> MRGSHHHHHHGMASEDRPIKFSTEGATSQSYKQFIEALRERLRGGLIHDIPVLPDPTTLQERNRYITVELSNSDTESIEVGIDVTNAYVVAYRAGTQSHFLRDAPSSASDYLFTGTDQHSLPFYGTYGDLERWAHQSRQQIPLGLQALTHGISFFRSGGNDNEEKARTLIVIIQMVAEAARFRYISNRVRVSIQT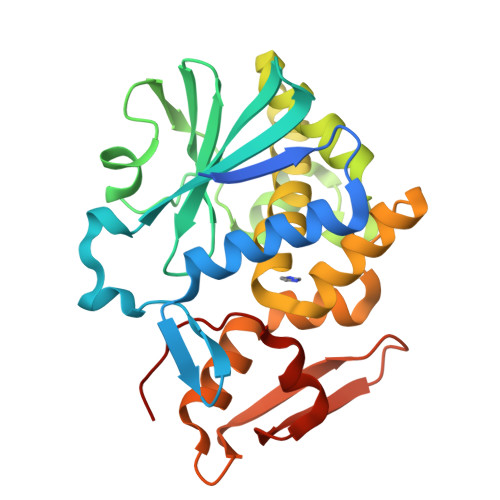GTAFQPDAAMISLENNWDNLSRGVQESVQDTFPNQVTLTNIRNEPVIVDSLSHPTVAVLALMLFVCNPPN> MSSLPVAAVLPELLTALDCAPQVLLSAPTGAGKSTWLPLQLLAHPGINGKIILLEPRRLAARNVAQRLAELLNEKPGDTVGYRMRAQNCVGPNTRLEVVTEGVLTRMIQRDPELSGVGLVILDEFHERSLQADLALALLLDVQQGLRDDLKLLIMSATLDNDRLQQMLPEAPVVISEGRSFPVERRYLPLPAHQRFDDAVAVATAEMLRQESGSLLLFLPGVGEIQRVQEQLASRIGSDVLLCPLYGALSLNDQRKAILPAPQGMRKVVLATNIAETSLTIEGIRLVVDCAQERVARFDPRTGLTRLITQRVSQASMTQRAGRAGRLEPGISLHLIAKEQAERAAAQSEPEILQSDLSGLLMELLQWGCSDPAQMSWLDQPPVVNLLAAKRLLQMLGALEGERLSAQGQKMAALGNDPRLAAMLVSAKNDDEAATAAKIAAILEEPPRMGNSDLGVAFSRNQPAWQQRSQQLLKRLNVRGGEADSSLIAPLLAGAFADRIARRRGQDGRYQLANGMGAMLDANDALSRHEWLIAPLLLQGSASPDARILLALLVDIDELVQRCPQLVQQSDTVEWDDAQGTLKAWRRLQIGQLTVKVQPLAKPSEDELHQAMLNGIRDKGLSVLNWTAEAEQLR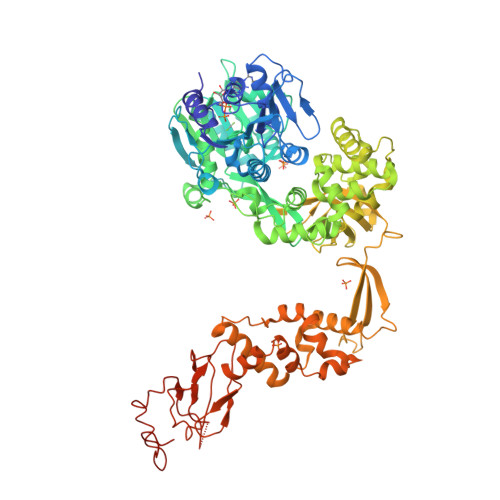LRLLCAAKWLPEYDWPAVDDESLLAALETWLLPHMTGVHSLRGLKSLDIYQALRGLLDWGMQQRLDSELPAHYTVPTGSRIAIRYHEDNPPALAVRMQEMFGEATNPTIAQGRVPLVLELLSPAQRPLQITRDLSDFWKGAYREVQKEMKGRYPKHVWPDDPANTAPTRRTKKYS>MALGPAAMGYDRAITIFSPDGSLYQVDYAFEAVKRGWTTLGVKTKSGVVLLAEKRKATQLLDVDGIEKIFMLDDHVGCTFAGLASDGRILIDYARSQALQHRLIYDEPISIEYLTKVISDVKQAYTQHGGVRPFGVALIVGGIDKGKQPKLLMTEPSGQFMPYYAVAIGQGGYTATEYLEKNYKEDLDIQSTILLALRALMATLKPGEKLNYSSVEIGYADVDSGTFKKLTTEERSDLLQKI[14x];>[14x]MTAIGIKTKDGVVLAAERRLSYGDFVLSKSARKVFKLGRFGIAGAGIVG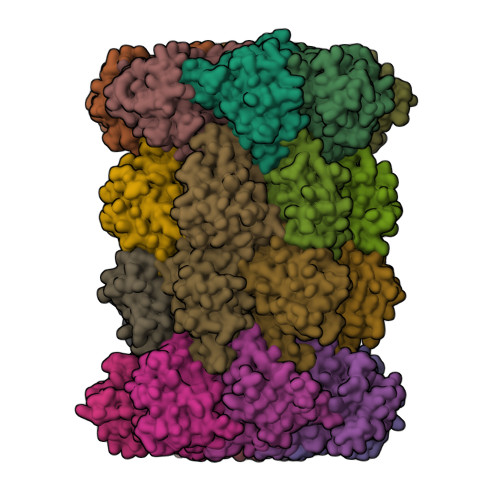DIQTLTRIMNVEIKYYEMYNSRKISARAAAKLLSVILYQNKVLPYISELLFGGVDEDGPKLFILDPIGSLIEDSYAAVGSGARVAIGVLEAEYNESLTSEAAKELAIKSMKSAVERDVMSGDGIDILIINKNNIYEDFIKILEHHHHHH>[16x]MKNLDINTFDNIEDIPLGSSEQDPYDFFTLSDRNVMNSDMKKNIVQWNSRYSYNQLKNKDSLIMFLVEIFRSLFVSNCIDKNIDNVLLSIEEMFIDHYYNPQHSRLKYLIDDVGIFFTKLPITKAFHTYNKKYRITKRLYAPPTFNEVRHILNLAQILSLEEGLDLLTFDADET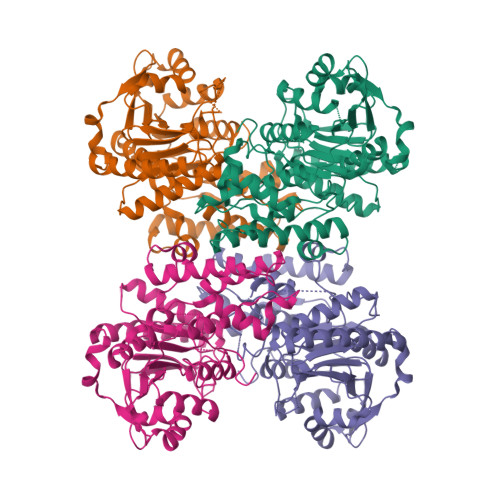LYPDGHDFNDEVLASYISCLLKKMNIAIVTAASYNNDAEKYQKRLENLLKYFSKHNIKDGSYKNFYVMGGESNYLFKCNEEATLYSVPENEWRHYKKFVDYDTVQEILNISEKCLEKVIKDFGLCAQIQRKEKSIGLVPNKIPSLNIKNEQKNYMIKYEVLEEAVIRIKKEIIKNKITAPYCAFNGGQDLWVDVGNKAEGLLILQKLLKIQKKKCCHIGDQFLHSGNDFPTRFCSLTLWVSNPQETKACLKSIMHLNIKSFIPEVLYENQ Neprosin from the pitcher plant is a reported prolyl endopeptidase. Here, we produce recombinant neprosin and its mutants, and find that full-length neprosin is a zymogen, which is self-activated at gastric pH by the release of an all-β pro-domain via a pH-switch mechanism featuring a lysine plug. The catalytic domain is an atypical 7+8-stranded β-sandwich with an extended active-site cleft containing an unprecedented pair of catalytic glutamates. Neprosin efficiently degrades both gliadin and the 33-mer in vitro under gastric conditions and is reversibly inactivated at pH > 5.

The final refined model of the derivative complex was used to solve the native pro-neprosin structure by molecular replacement. Moreover, mature neprosin produced two different monoclinic crystal forms, I and II, whose structures were likewise solved by molecular replacement. The structure of mature neprosin crystal form I proved practically identical to the equivalent part of the zymogen, with a core root mean square deviation (RMSD) of 0.62 Å. The only significant difference was encountered at N232–Y233, which is folded outward in the zymogen to accommodate I103 at the beginning of the rightmost strand of the PD. Moreover, in the structures of mature neprosin crystal forms I and II, the C-terminal segment, which spanned an alanine–isoleucine–alanine tripeptide followed by the His6-tag, ran along the surface of a symmetry mate, thus mimicking a product complex. Both crystal forms were monoclinic but with different cell constants, which resulted in variable crystal packing. Even so, the C-terminal tag penetrates the cleft in a similar manner in both crystallographic arrangements but is shifted by three positions, so that H404–H409 from crystal form I overlaps A401–H406 from crystal form II. Indeed, we found a striking pair of glutamate residues (E188 and E297) bridged by a solvent molecule pinching the bound peptides in the product complexes. Our results suggest that the mature neprosin structures mimic upstream product complexes collectively occupying subsites S6 to S1′, with the two catalytic glutamates plus the bridging solvent molecule poised for reaction.

> SANTNHQYAVIAYFYGNASLQGANATINIWEPNLKNPNGDFSLTQIWISAGSGSSLNTIEAGWQVYPGRTGDSQPRFFIYWTADGYTSTGCYDLTCPGFVQTNNYYAIGMALQPSVYGGQQYELNESIQRDPATGNWWLYLWGTVVGYWPASIYNSITNGADTVEWGGEIYDSSGTGGFHTTTQMGSGHFPTEGYGKASYVRDLQCVDTYGNVISPTANSFQGIAPAPNCYNYQFQQGSSELYLFYGGPGCQAIAHHHHHH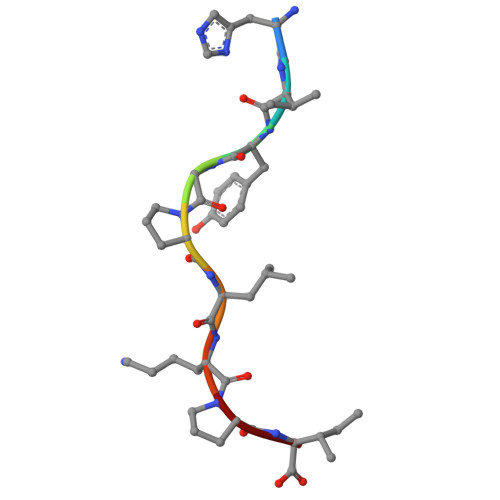> HVYGPLKPI> MVSSDRPVSLEDEVSHSMKEMIGGCCVCSDERGWAENPLVYCDGHGCSVAVHQACYGIVQVPTGPWFCRKCESQERAARVRCELCPHKDGALKRTDNGGWAHVVCALYIPEVQFANVSTMEPIVLQSVPHDRYNKTCYICDEQGRESKAATGACMTCNKHGCRQAFHVTCAQF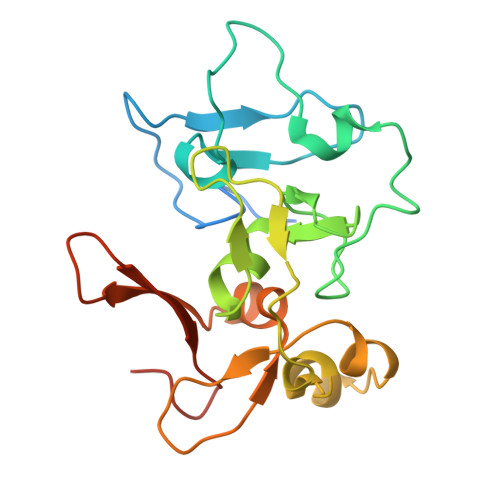AGLLCEEEGNGADNVQYCGYCKYHFSKLKKSKRGS> MEIPVIEPLFTKVTEDIPGAAGPVFDKNGDFYIVAPYVEVNGKPAGEILRIDLKTGKKTVICKPEVNGYGGIPIGCQCDRDANQLFVADMRLGLLVVQTDGTFEEIAKKDSEGRRMQGCAYCAFDYEGNLWITAPAGEVAPADFTISLQEKFGSIYCFTTDGQMIQVDTAFQAPAGIAVRHMNDGRPYQLIVAEQPTKKLWSYDIKGPAKIENKKVWGHIPGTHKGGAAGMDFDEDNNLLVANWGSSHIEVFGPDGGQPKMRIRCPFEKPSALHFKPQTKTIFVTEHENNAVWKFEWQRNGKKQY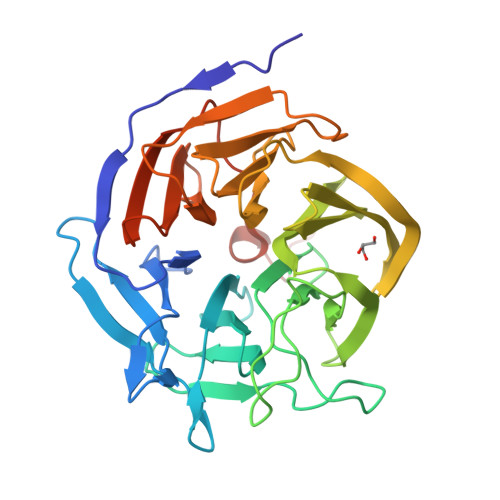CETLKFGIFGSLEHHHHHH>[2x]GSHMEEKLAVSLQEALQEGDTRALREVLEEIHPQDLLALWDELKGEHRYVVLTLLPKAKAAEVLSHLSPEEQAEYLKTLPPWRLREILEELSLDDLADALQAVRKEDPAYFQ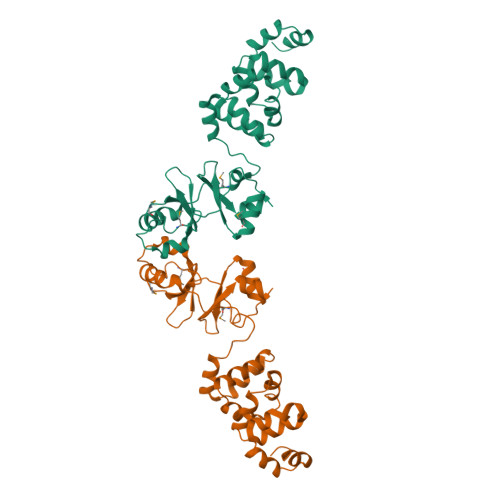RLKDLLDPRTRAEVEALARYEEDEAGGLMTPEYVAVREGMTVEEVLRFLRRAAPDAETIYYIYVVDEKGRLKGVLSLRDLIVADPRTRVAEIMNPKVVYVRTDTDQEEVARLMADYDFTVLPVVDEEGRLVGIVTVDDVLDVLEAEATEDIHKLGAVDVPDLVYSE> MNADEWMTTFRENIAQTWQQPEHYDLYIPAITWHARFAYDKEKTDRYNERPWGGGFGLSRWDEKGNWHGLYAMAFKDSWNKWEPIAGYGWEST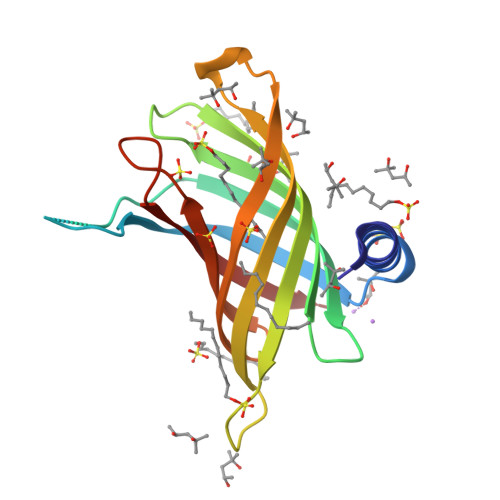WRPLADENFHLGLGFTAGVTARDNWNYIPLPVLLPLASVGYGPVTFQMTYIPGTYNNGNVYFAWMRFQFL>[3x]LPRETDEEPEEPGKTGSFVEMVDNLRGKSGQGYYVEMTVGSPPQTLNILVDTGSSNFAVGAAPHPFLHRYYQRQLSSTYRDLRKGVYVPYTQGKWEGELGTDLVSIPHGPNVTVRANIAAITESDKFFINGSNWEGILGLAYAEIARPDDSLEPFFDSLVKQTHVPNLFSLQLCGAGFPLNQSEVLASVGGSMIIGGIDHSLYTGSLWYTPIRREWYYEV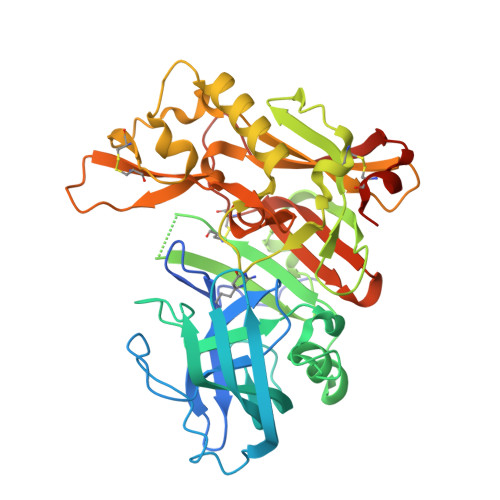IIVRVEINGQDLKMDCKEYNYDKSIVDSGTTNLRLPKKVFEAAVKSIKAASSTEKFPDGFWLGEQLVCWQAGTTPWNIFPVISLYLMGEVTNQSFRITILPQQYLRPVEDVATSQDDCYKFAISQSSTGTVMGAVIMEGFYVVFDRARKRIGFAVSACHVHDEFRTAAVEGPFVTLDMEDCGYNIPQTDES> KEINFDDD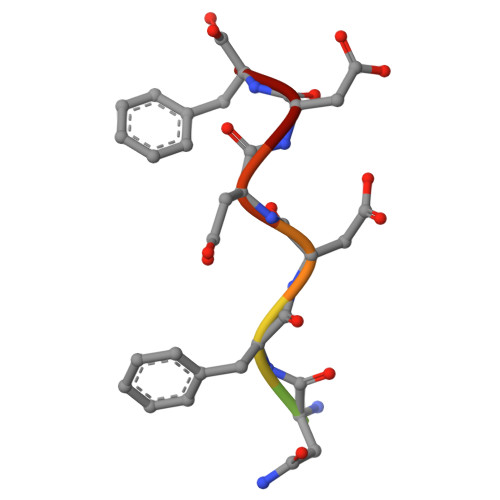F> DPH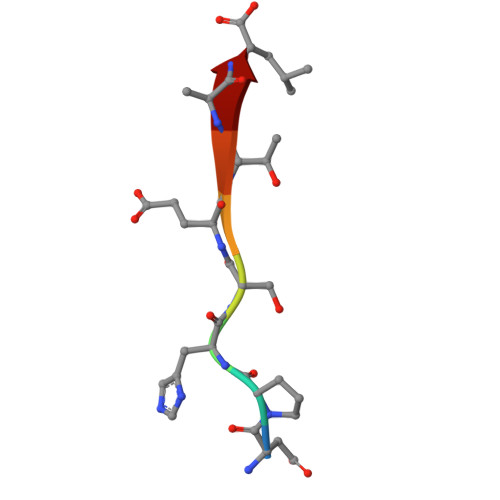SETAL>VSEDLRSRIEVLKRKVIEKVQHIQLLQKNVRAQLVDMKRLEVDIDIK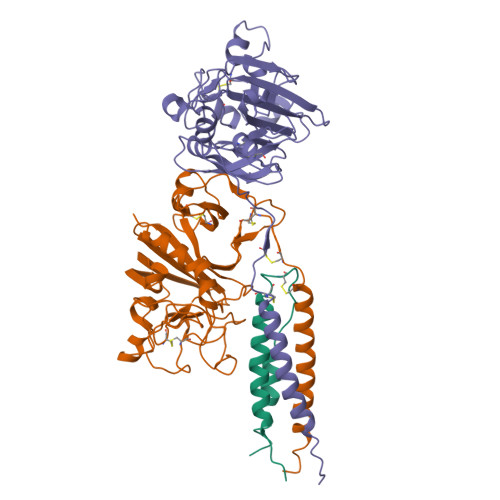IRSCRGSCSRALAREVDLKDYEDQQKQLEQVIAKDLLPSR[2x];>[2x]DNENVVNEYSSELEKHQLYIDETVNSNIPTNLRVLRSILENLRSKIQKLESDVSAQMEYCRTPCTVSCNIPVVSGKECEEIIRKGGETSEMYLIQPDSSVKPYRVYCDMNTENGGWTVIQNRQDGSVDFGRKWDPYKQGFGNVATNTDGKNYCGLPGEYWLGNDKISQLTRMGPTELLIEMEDWKGDKVKAHYGGFTVQNEANKYQISVNKYRGTAGNALMDGASQLMGENRTMTIHNGMFFSTYDRDNDGWLTSDPRKQCSKEDGGGWWYNRCHAANPNGRYYWGGQYTWDMAKHGTDDGVVWMNWKGSWYSMRKMSMKIRPFFPQQ;>[2x]KMLEEIMKYEASILTHDSSIRYLQEIYNSNNQKIVNLKEKVAQLEAQCQEPCKDTVQIHDITGKDCQDIANKGAKQSGLYFIKPLKANQQFLVYCEIDGSGNGWTVFQKRLDGSVDFKKNWIQYKEGFGHLSPTGTTEFWLGNEKIHLISTQSAIPYALRVELEDWNGRTSTADYAMFKVGPEADKYRLTYAYFAGGDAGDAFDGFDFGDDPSDKFFTSHNGMQFSTWDNDNDKFEGNCAEQDGSGWWMNKCHAGHLNGVYYQGGTYSKASTPNGYDNGIIWATWKTRWYSMKKTTMKIIPFNRLTIGEGQQHHLGGAK;>[2x]MVNGDGNPREVIEDLAANNPAIQNIRLRHENKDLKARLENAMEVAGRDFKRAEELEKAKQALEDQRKDLETKLKELQQDYDLAKESTSWDRQRLEKHHHHHH>MSERAYNFNAGPAALPLEVLERAQAEFVDYQHTGMSIMEMSHRGAVYEAVHNEAQARLLALLGNPTGYKVLFIQGGASTQFAMIPMNFLKEGQTANYVMTGSWASKALKEAKLIGDTHVAASSEASNYMTLPKLQEIQLQDNAAYLHLTSNETIEGAQFKAFPDTGSVPLIGDMSSDILSRPFDLNQFGLVYAGAQKNLGPSGVTVVIVREDLVAESPKHLPTMLRYDTYVKNNSLYNTPPSFGIYMVNEVLKWIEERGGLEGVQQANRKKASLIYDAIDQSGGFYRGCVDVDSRSDMNITFRLASEELEKEFVKASEQEGFVGLKGHRSVGGLRASIYNAVPYESCEALVQFMEHFKRSR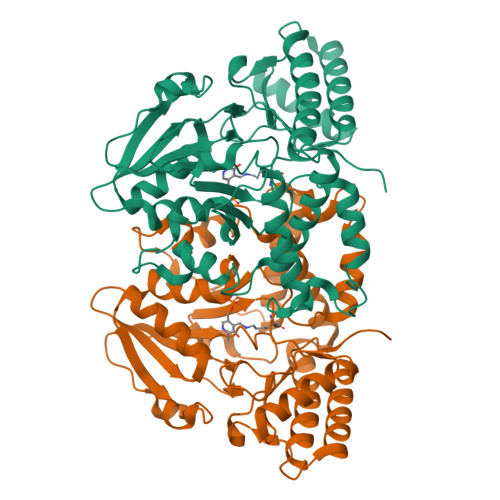G[2x]> MRPEVEQELSHVLLTELLAYQFASPVRWIETQDVFLKDYNTERVVEIGPSPTLAGMASRTIKAKYESYDAALSLQRQVLCYAKDTKEIYYTPDPADIAPPIKEEAETSAAATSSSAPAAAAPVSAAPAAAPSGPVAEIPDEPVKAALVLHVLVAHKLKKSLDAVPLSKAIKDLVGGKSTVQNEILGDLGKEFGSTPEKPEDTPLQELAEQFQDTFPGSLGKQTGSLVNRLMSSKMPGGFSLSVARKYLQTRWGLGPGRQDSVLLVALVNEPGARLSSDGEAKEFLDSCAQKYASGAGITLAQAAAGGAGSSGAGGAVIDAEAFEELTKDNRVLARQQLEVLARYLKYDLTKGEKSLVKEKEASSLLQQELDLWAEEHGEIYAQGIKPVFSHLKARTYDSYWNWARQDALSMYFDIIFGKLTDVDRETVSQCIQLMNRSNPTLIKFMQYHIDHCPEYKGETYQLAKSLGQQLIDNCIQVANQDPVYKDISYPTGPHTEVDSKGNIVYKEVNRKSVRKLEQYVFEMSQGGELTKEVQPTIQEDLAKIYEALNKQASTESQLEFNKLYNSLIEFVEKSKEIEVSKSINAVLASKSSDSDRSAEISSLSEKTSIVDPVSGGIPPETVPFLHLKKKLPSGEWVFDRDTSALFLDGLQKGAVNGISYKGKNVLITGAGAGSIGAEVLQGLISGGAKVIVTTSRFSKKVTEYYQDIYARFGAAGSCLIVVPFNQGSKQDVEALIDYIYRDVKDEGLGWDLDAVIPFAAIPEAGIEIDELGSKSELAHRIMLTNLLRLLGEVKKQKFTRAINTRPAQIILPLSPNHGTFGSDGLYSESKLGLETLFNRWYSESWSEQLTVCGAIIGWTRGTGLMSGNNIIAEGLEKLGVRTFSQKEMAFNILGLMTPELTEMCQNGPVVADLNGGLQFIENLREYTAQLRNEIYETSEVRRAVSIETGIETRVVNGENADAPYQKARIEPRANLKFEFPPLKSHKEIQNKAPGLEGLLDLERVIVVTGFGEVSPWGNTRTRWEMEAFGEFSIEGCLEMAWIMGFIKYHNGNLKGKPYTGWIDAKTNEPVEDKDIKKKYEEEILAHAGIRLIEPELFRGYNPEKKELIQEVIIEQDMAPFVTDESTAQQYKLQHEDAVDILKSEESDEYTVTFKKGARLFVPKALRFDRLVAGQIPTGWDAKRYGISEDTISQVDPVTLYALVSTIEALLSAGITDPYEFYKYVHVSEVGNCSGSGMGGVSALRGMFRDRYSDKPVQNDILQESFINTMSAWVNMLLLSSSGPIKTPVGACATAVESVDIGVETILSGKAKICLVGGYDDFQEEGSYEFANMNATSNSLDEFDHGRTPQEMSRPATTTRNGFMEAQGSGTQVIMNAELAIKMGVPIYAIVALTATATDKIGRSVPAPGKGILTTAREHHGSLKTKSPKLDIKYRTRQLNKR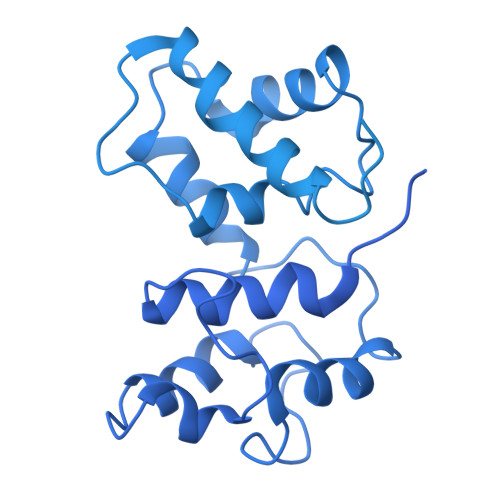KDQIKQWVEDELEYIREEAAELANSDAKFDAVSFVSERTEEVYREATKQVKMAQQEWGNEFWKNDPRIAPLRGALATFNLTVDDLGVASFHGTSTKANDKNESITINKMMQHLGRSEGNPVFGVFQKYLTGHPKGAAGAWMLNGAIQILQTGIVPGNRNADNVDKILEDFEYVLYPSRSIQTDGIKACSVTSFGFGQKGGQAIVVHPDYLFASLDSETFEEYKTKVEARYKSTYRYMHNAIIRNTMFVAKSDPPYTDELEQPVYLDPLARVNNCKKNPSKLVFVNADVQSKQNFVGKSANDTAKVISSLTSDVTSGGKGVGVDVELISAINNENHTFIERNFTENEISYCASAPSSKSSLAGTWSAKEAVFKALGVESKGAGASLKDIEIVRDSKGAPTVVLHGDAKSAASAAGVKNVKVSISHDDVQSVAVAISEF>[4x]DGENLRPVVIDGSNVAMSHGNKEVFSCRGIKLAVDWF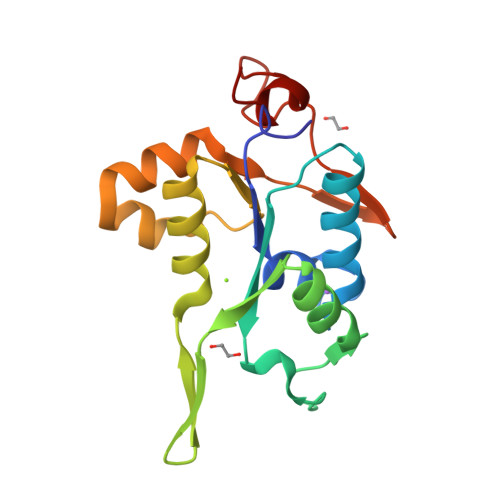LERGHKDITVFVPAWRKEQSRPDALITDQEILRKLEKEKILVFTPSRRVQGRRVVCYDDRFIVKLAFESDGIIVSNDNYRDLANEKPEWKKFIDERLLMYSFVNDKFMPPDDPLGRHGPSLDNFLRKK> GSSGSSGMGKRLDLSTLTDEEAEHVWAVVQRDFDLRRREEERLQGLKGKIQKESSKRELLSDTAHLNETHCARCLQPYRLLLNSRRQCLECSLFVCKSCSHAHPEEQGWLCDPCHLARVVKIG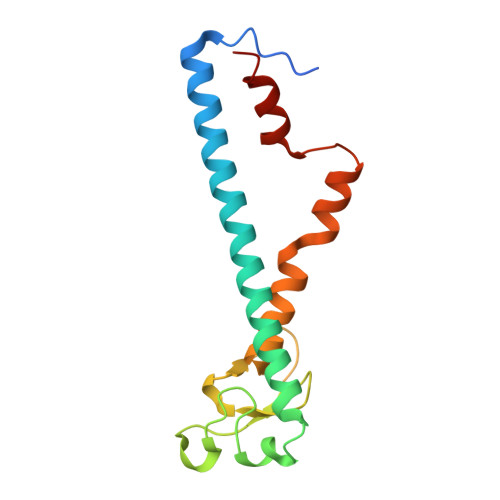SLEWYYQHVRARFKRFGSAKVIRSLCGRLQ>ADDALAALGAQLFVDPALSRNATQSCATCHDPARAFTDPREGKAGLAVSVGDDGQSHGDRNAPTLGYAALVPAFHRDANGKYKGGQFWDGRADDLKQQAGQPMLNPVEMAMPDRAAVAARLRDDPAYRTGFEALFGKGVLDDPERAFDAAAEALAAYQATGEFSPFDSKYDRVMRGEEKFTPLEEFGYTVFITWNCRLCHMQRKQGVAERETFTNFEYHNIGLPVNETAREASGLGADHVDHGLLARPGIEDPAQSGRFKVPSLRNVAVTGPYMHNGVFTDLRTAILFYNKYTSRRPEAKINPETGAPWGEPEVARNLSLAELQSGLMLDDGRVDALVAFLETLTDRRYEPLLEE[2x];>[2x]TDPRAKWVPQDNDIQACDYWRHCSIDGNICDCSGGSLTNCPPGTKLATASWVASCYNPTDGQSYLIAYRDCCGYNVSGRCPCLNTEGELPVYRPEFANDIIWCFGAEDDAMTYHCTISPIVGKAS;>[2x]QETQGQAAARAAAADLAAGQDDEPRILEAPAPDARRVYVNDPAHFAAVTQQFVIDGEAGRVIGMIDGGFLPNPVVADDGSFIAHASTVFSRIARGERTDYVEVFDPVTLLPTADIELPDAPRFLVGTYPWMTSLTPDGKTLLFYQFSPAPAVGVVDLEGKAFKRMLDVPDCYHIFPTAPDTFFMHCRDGSLAKVAFGTEGTPEITHTEVFHPEDEFLINHPAYSQKAGRLVWPTYTGKIHQIDLSSGDAKFLPAVEALTEAERADGWRPG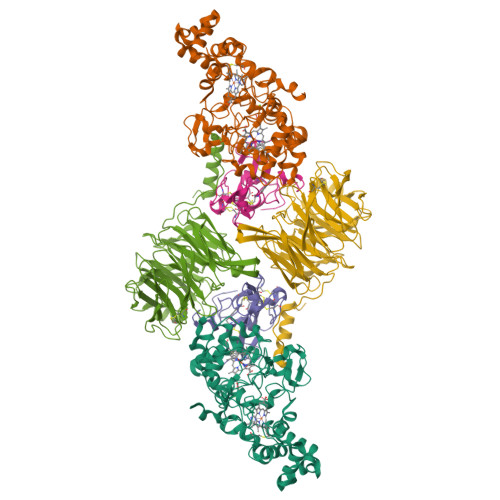GWQQVAYHRALDRIYLLVDQRDEWRHKTASRFVVVLDAKTGERLAKFEMGHEIDSINVSQDEKPLLYALSTGDKTLYIHDAESGEELRSVNQLGHGPQVITTADMG> GSMQANQWQSVQNRTFTKWFNTKLSSRDLPSVFDLRKDLSDGILLIQLLEIIGDENLGRYNRNPRMRVHRLENVNKALEYIKSKGMPLTNIGPADIVDGNLKLILGLIWTLILRFTIADINEEGLTAK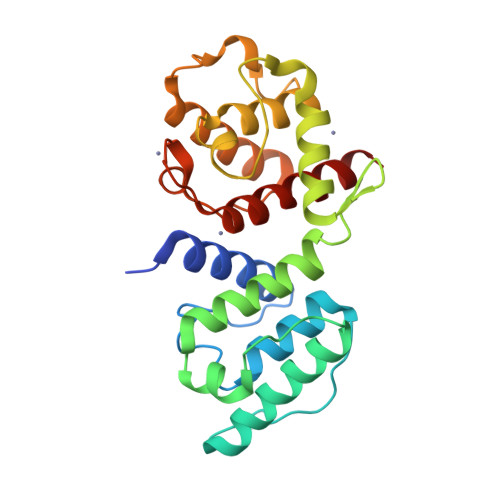EGLLLWCQRKTANYHPEVDVQDFTRSWTNGLAFCALIHQHRPDLLDYNKLDKKNHRANMQLAFDIAQKSIGIPRLIEVEDVCDVDRPDERSIMTYVAEYFHAFSTLDK> ARGSHMEEMIRSLQQRPEPTPEEWDLIHIATEAHRSTNAQGSHWKQRRKFLPDDIGQSPIVSMPDGDKVDLEAFSEFTKIITPAITRVVDFAKKLPMFSELPCEDQIILLKGCCMEI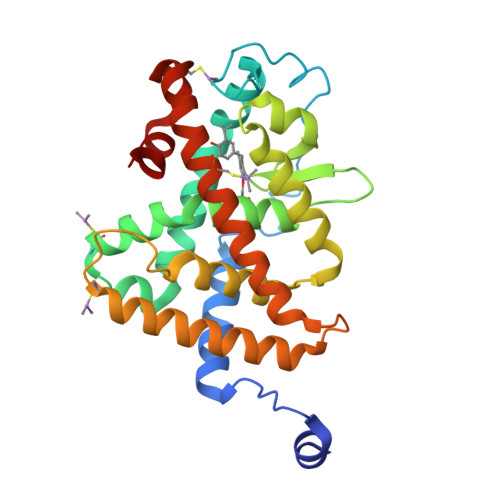MSLRAAVRYDPESDTLTLSGEMAVKREQLKNGGLGVVSDAIFELGKSLSAFNLDDTEVALLQAVLLMSTDRSGLLCVDKIEKSQEAYLLAFEHYVNHRKHNIPHFWPKLLMKVTDLRMIGACHASRFLHMKVECPTELFPPLFLEVFEDQEV>[2x]SMLKLSAENESTPIQQLLEHFLRQLQRKDPHGFFAF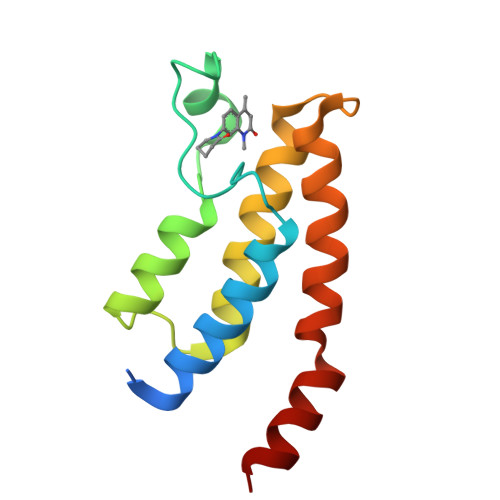PVTDAIAPGYSMIIKHPMDFGTMKDKIVANEYKSVTEFKADFKLMCDNAMTYNRPDTVYYKLAKKILHAGFKMMSKERLLALKRSMS>[2x]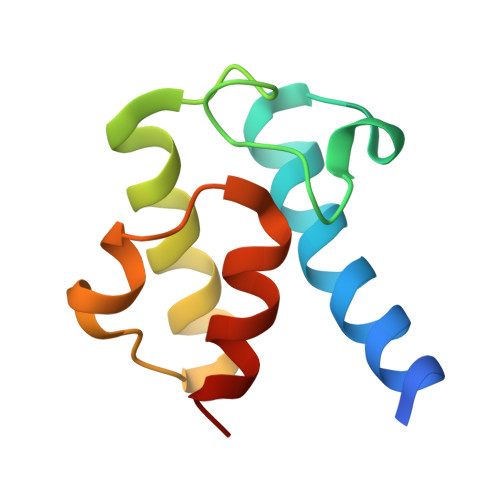AMGYLAMGYLMALFEDIQAVIAEQLNVDAAQVTPEAEFVKDLGADSLDVVELIMALEEKFGIEIPDEQAEKIVNVGDVVKYIEDNKLA2-[[5-chloranyl-2-[[4-[[[1-[2-(propanoylamino)ethyl]-1,2,3-triazol-4-yl]methylamino]methyl]phenyl]amino]pyrimidin-4-yl]amino]-~{N}-methyl-benzamide | C27 H31 Cl N10 O2 | 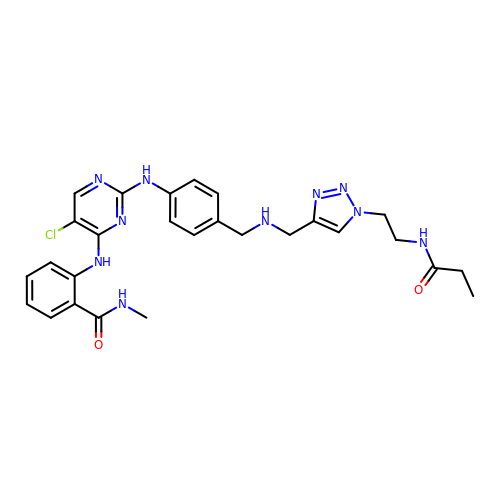NQZYJQAUOJXIDJ-UHFFFAOYSA-N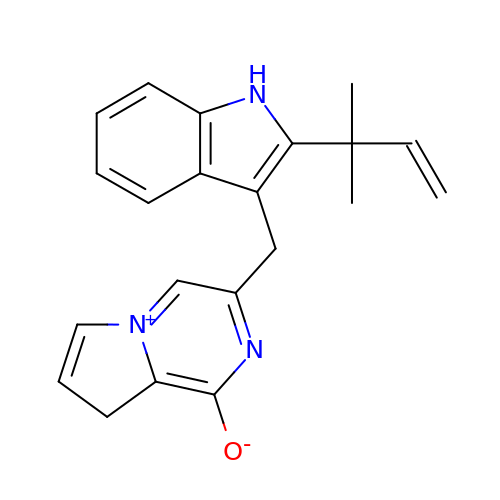3-{[2-(2-methylbut-3-en-2-yl)-1H-indol-3-yl]methyl}-8H-pyrrolo[1,2-a]pyrazin-5-ium-1-olate | C21 H21 N3 O | DUPBTPHDPVCZPP-UHFFFAOYSA-N> GAMGSMSKQFVRSAKNLVKGYSSTQVLVRNATSNDNHQVSKDSLIELAEKSYDSADFFEIMDMLDKRLNDKGKYWRHIAKALTVIDYLIRFGSENCVLWCRENLYIIKTLKEFRHEDDEGIDQGQIVRVKAKELTALLSDDERLNEERNMNIKGR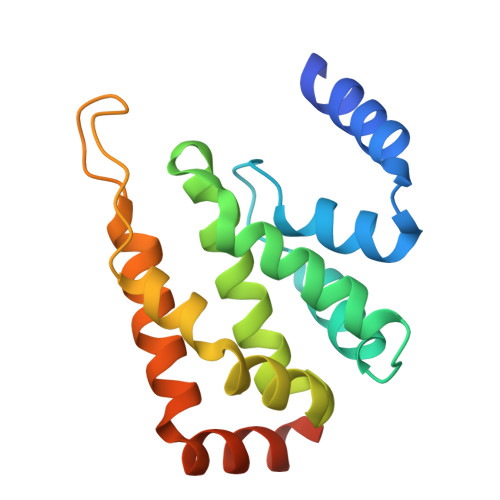NRKGRRR3,5-dichloro-N-(8-fluoroisoquinolin-5-yl)-2-hydroxybenzene-1-sulfonamide 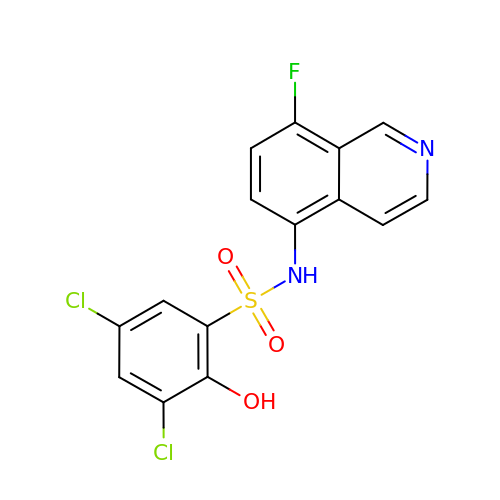| C15 H9 Cl2 F N2 O3 S | WUOPNKAKZGINIW-UHFFFAOYSA-N>HMTELLKNHVAGQWIAGTGAGITLTDPVTGVALVRVSSEGLDLARAFSFAREDGGAALRALTYAQRAARLADIVKLLQAKRGDYYAIATANSGTTRNDSAVDIDGGIFTLSYYAKLGASLGEVHALRDGSAESLSKDRSFSAQHVLSPTRGVALFINAFNFPSWGLWEKAAPALLSGVPVIVKPATATAWLTQ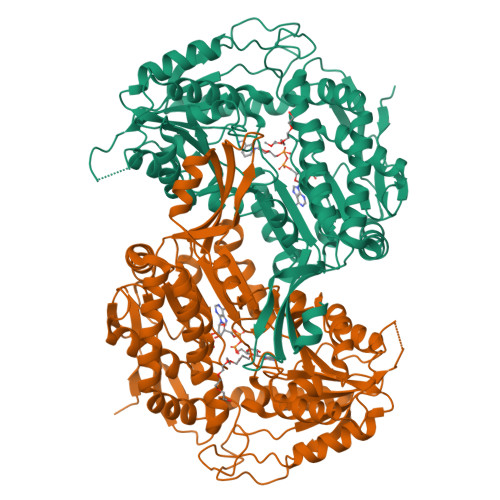RMVADVVDAGILPPGALSIICGSSAGLLDQIRSFDVVSFTGSADTAATLRAHPAFVQRGARLNVEADSLNSAILCADATPDTPAFDLFIKEVVREMTVKSGQKCTAIRRAFVPEAALEPVLEALKAKLAKITVGNPRNDAVRMGSLVSREQYENVLAGIAALREEAVLAYDSSAVPLIDADANIAACVAPHLFVVNDPDNATLLHDVEVFGPVASVAPYRVTTDTNALPEAHAVALARRGQGSLVASIYSNDDAHLGRLALELADSHGRVHAISPSVQHSQTGHGNVMPMSLHGGPGRAGGGEELGGLRALAFYHRRSAIQAASAAIGTLTQATHWPAA[2x]>MSKLPFLSRAAFARITTPIARGLLRVGLTPDVVTILGTTASVAGALTLFPMGKLFAGACVVWFFVLFDMLDGAMARERGGGTRFGAVLDATCDRISDGAVFCGLLWWIAFHMRDRPLVIATLICLVTSQVISYIKARAEASGLRGDGGFIERPERLIIVLTGAGVSDFP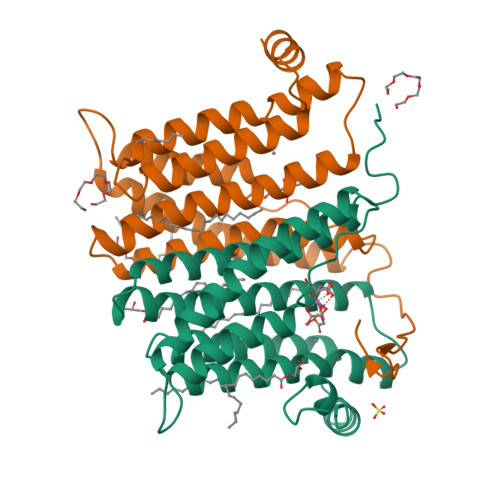FVPWPPALSVGMWLLAVASVITCVQRLHTVWTSPGAIDRMAIPGKGDRENLYFQ[2x]>[2x]MDTSLAEEVQQTMATLAPNRFFFMSP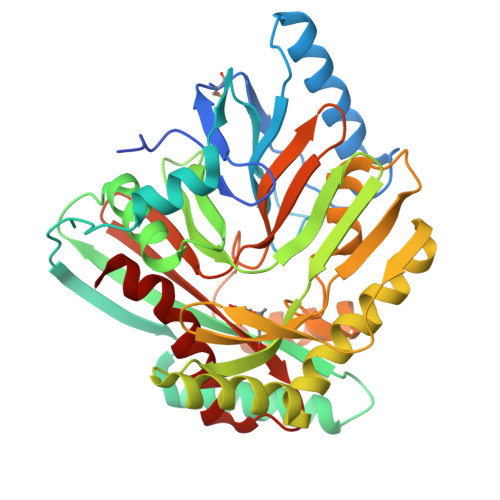YRSFTTSGCFARFDEPAVNGDSPDSPFQQKLAALFADAKAQGIKNPVMVGAIPFDPRQPSSLYIPESWQSFSRQEKQASARRFTRSQSLNVVERQAIPEQTTFEQMVARAAALTATPQVDKVVLSRLIDITTDAAIDSGVLLERLIAQNPVSYNFHVPLADGGVLLGASPELLLRKDGERFSSIPLAGSARRQPDEVLDREAGNRLLASEKDRHEHELVTQAMKEVLRERSSELHVPSSPQLITTPTLWHLATPFEGKANSQENALTLACLLHPTPALSGFPHQAATQVIAELEPFDRELFGGIVGWCDSEGNGEWVVTIRCAKLRENQVRLFAGAGIVPASSPLGEWRETGVKLSTMLNVFGLH> GVFEELAAGQQRKYIMISGKGGVGKTSLSASLAVKLAAAGHTTLVVSTDPAHSLSDSLAQDVSGGRPVLLQGTDLPLWGLEIDPEEAKREFFEGSGAGQDGEAGGPSAASQVSDFMNRMGMGFVIDQLKELKLGELLNTPPPGLDEAVAIAKVVQFVQAAEYARFSRIVFDTAPTGHTLRLLALPDFVDASLAKVIRLRKKLNGATSVVRGLFGAGESQDEAVEKLELLQQRVRMVKALFRDKTQTEFIIATIPTYLGVNESSRLLQALRAEQIPCKRIIVNQIVGPQQGDAYLRMKMKDQIAALEMVANDPGLRPLRKVIAPMVDVEVRGVPALSYFGNVVWKDVYDQMNQGADRKFFLLGGKGGVGKTSCSSSLAVHFANDGLPTLVVSTDPAHSLSDAFDQDLSGGSPVKITSPLGDELPLWGLQLDPEQAKAELRAVLADDGGKKLNETLDGLGLGVISDQLKDLQLGELLDTPPPGVDEAI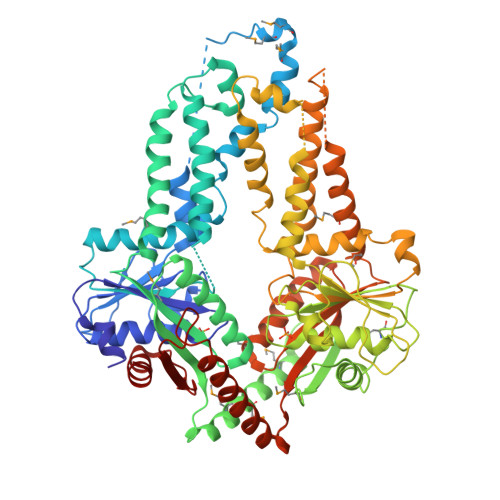AIAKVVQFLKAPEYSHFKRIVFDTAPTGHTLRLLSLPDFLDASIGKLVRLRQKLSAATSAVKNLFSGGQPGEEDVAVKRLEALQASMEDAKAMFRNQQTTEFIIVTIPTVMATAESCRLASALQHEGIPLKTIIVNQVVQANATDKFLTARRADQARALHHLEEDTGPDGLASLQLIKAPLCDLEVRGVPALSYFGNVVWK We aimed to develop covalent inhibitors targeting tyrosine residues in the protein kinases JAK3 and MK2 using structure-based design principles to generate small sets of ligands containing tyrosine-reactive sulfonyl fluoride and the less-explored fluorosulfate warheads. By utilizing a structure-based approach with well-characterized kinases, we focus on Janus kinase 3 (JAK3) and mitogen-activated protein kinase-activated protein kinase 2 (MK2, also known as MAPKAPK2) as model targets. In conclusion, we successfully synthesized a small but diverse set of novel fluorosulfate and sulfonyl fluoride warhead-bearing compounds, initially designed to covalently target tyrosine residues in both JAK3 and MK2 using structure-based design principles.

JAK3, a member of the Janus kinase family, is pivotal in the signaling pathways of common gamma chain (γc) cytokine receptors. We therefore hypothesized that replacing the cyano group by a fluorosulfate (or sulfonyl fluoride) warhead along with a conformational flip of the phenyl moiety could lead to the first tyrosine-targeting covalent inhibitor of JAK3. Only molecule 25a bearing the sulfonylfluoride warhead in meta position showed an IC50 of 26 nM, close to the inhibitory activity of our non-covalent design starting point (IC50 = 5.2 nM). To validate potential covalent interactions, we performed intact protein mass spectrometry (MS) experiments (3-fold excess compound over JAK3, 4 °C due to stability issues of the JAK3 enzyme, 24 h) to verify whether any of our compounds actually form a covalent bond with the target. Unfortunately, no mass shift as a result of covalent bond formation was observed, indicating that none of the molecules bound covalently to JAK3. We hypothesized that while inhibitor 25a shows nanomolar inhibitory activity, it likely orients itself in the same way as our non-covalent design template 6 where the nitrile points away from the target tyrosine, and therefore the warhead is solvent-exposed rather than pointing towards the hinge region where the target tyrosine is located. We validated this hypothesis by solving the X-ray crystal structure of 25a in complex with JAK3. This crystal structure explains why there is no covalent bond formation – 25a indeed orients itself in exactly the same way that starting point 6 does. While we provide new structural insights into JAK3 inhibitor binding, the JAK3 inhibitors we designed did not achieve covalent binding to the hinge tyrosine side chain.

>[2x]SMQDPTIFEERHLKYISQLGKGNFGSVELCRYDPLGDNTGALVAVKQLQHSGPDQQRDFQREIQILKALHSDFIVKYRGVSYGPGRQSLRLVMEYLPSGCLRDFLQRHRARLDASRLLLYSSQICKGMEYLGSRRCVHRALAARNILVESEAHVKIADFGLAKLLPLDKDYYVVREPGQSPIFWYAPESLSDNIFSRQSDVWSFGVVLYELFTYCDKSCSPSAEFLRMMGSERDVPALSRLLELLEEGQRLPAPPACPAEVHELMKLCWAPSPQDRPSFSALGPQLDMLWSGSR>MAPKSKTTSASSSKITPGQMQENTVLLGSGSKLKAIKLTNVVNGKLTHPETSDLKPIDVEVQAFTSASQNISNFTLHKYRNICHVDTCAAHLSKSKENKEKLQARNLRLIVSSNEFLVVVKELNDSTVDNVVSFNKACAIMSAGVLKHTFDEEFDWKLSKYVKTNNTTKVIPDVKIINRLAGQMGLSAGNPYYWMIVPGYEFLYELYPAEVLAYTLVRLQYRKNLNIPDSMTDADIVSSLVMKMNRIHKLEQTSFDEALNLIGKDNVSEAYVELARDIGSTSKTKRNDEAILKFRELIASFLPALEADRIASAHV[4x]

Like all bunyaviruses, FMV has a segmented, negative-sense, single-stranded RNA (ssRNA) genome that is encapsulated by the viral nucleoprotein (N). Here, we present high-resolution crystal structures of FMV N in its RNA-free and RNA-bound forms, revealing a “paper fortune teller” structural transition between the two states. In general, N proteins of bunyaviruses consist of a globular core that includes the RNA binding cleft and two terminal arms (N and C arms) that enable oligomerization. The N protein serves as the main building block for the RNP assembly, protects the viral genome from endo- and exonucleases, and helps to evade the host’s innate immune response.

The trypsin-treated N protein (NΔN45) was then purified and screened for crystallization conditions. Finally, the structure was refined against a 2.28-Å-resolution data set with excellent statistics. The crystal structure of RNA-free NΔN45 revealed four NΔN45 molecules in the asymmetric unit that were organized in a tight tetramer, as was previously reported for N proteins from other members of the Bunyavirales order. Each of the monomers comprised an N-terminal arm (N arm, residues 52 to 71), a globular core (residues 71 to 280), and an α-helical C-terminal arm (C arm, residues 281 to 313). The N arm was mostly a coiled loop that contained a short β-strand (strand A), followed by the N-terminal subdomain (N lobe) of the globular core, which encompassed three α-helices (α1 to α3), and the BCD β-sheet, which was inserted between α2 and α3. The C-terminal subdomain of the core (C lobe) consisted of helices α4 through α10 and was followed by the C arm, a 33-residue-long amphipathic α-helix. The putative RNA binding cleft, a positively charged trench, was formed between the N and C lobes, and as expected, it did not contain any RNA molecules. Interestingly, unlike other bunyaviruses’ nucleoproteins, the FMV N presented one disulfide bond between C82 and C87 that was observed in all four copies of the asymmetric unit (bottom). The FMV N tetramer was organized as two dimers with 2-fold symmetry rather than having a 4-fold symmetry. Each protomer (N0) interacted with two other protomers via its N arm, which interacted with the N−1 protomer, and its C arm, which interacted with the N+1 protomer.> MKPHPWFFGKIPRAKAEEMLSKQRHDGAFLIRESESAPGDFSLS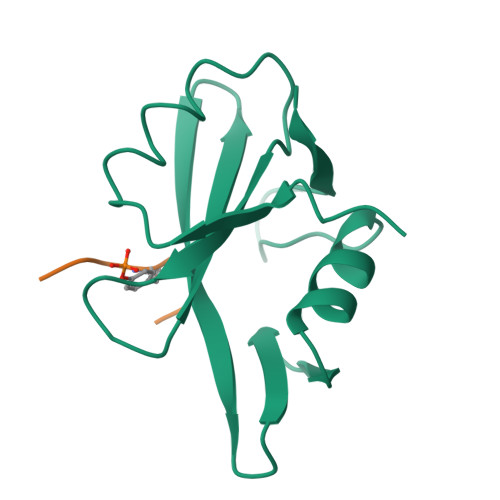VKFGNDVQHFKVLRDGAGKYFLWVVKFNSLNELVDYHRSTSVSRNQQIFLRDIE;> KPFYVNVX> MGSDKIHHHHHHMPTPADDLVVIGKIVSVYGIRGEVKVYSFTDPLDNLLDYRRWTLRRDGEIRQAELVRGRLHGKVLAAKLKGLDDREEARTFTGYEICI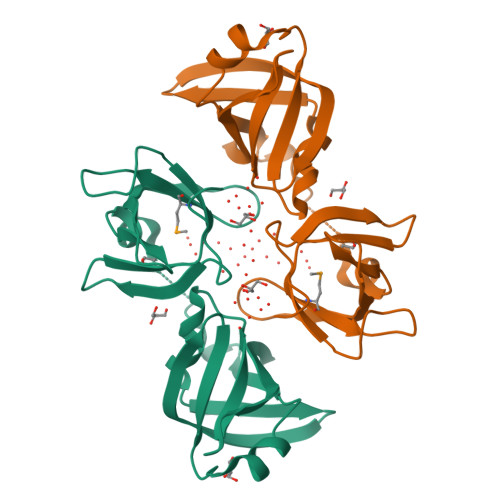PRSELPSLEEGEYYWHQLEGLKVIDQGRQLLGVIDHLLETGANDVMVVKPCAGSLDDRERLLPYTGQCVLSIDLAAGEMRVDWDADF> 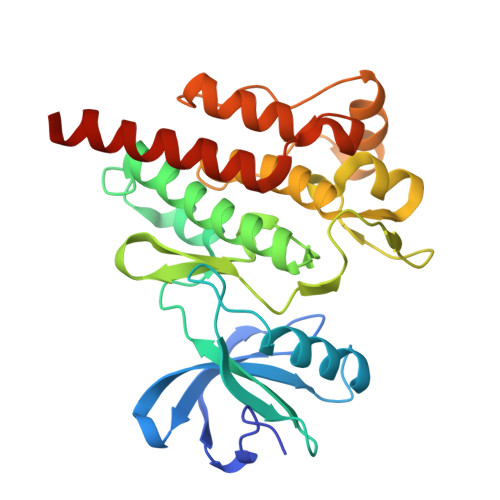GHMSPNYDKWEMERTDITMKHKLGGGQYGEVYEGVWKKYSLTVAVKTLKEDTMEVEEFLKEAAVMKEIKHPNLVQLLGVCTREPPFYIITEFMTYGNLLDYLRECNRQEVNAVVLLYMATQISSAMEYLEKKNFIHRDLAARNCLVGENHLVKVADFGLSRLMTGDTYTAPAGAKFPIKWTAPESLAYNKFSIKSDVWAFGVLLWEIATYGMSPYPGIDLSQVYELLEKDYRMERPEGCPEKVYELMRACWQWNPSDRPSFAEIHQAFETMFQESSISDEVEKELGK>ASAKLPGDFGPPRGEPIHAVLTSPPLVPPPVNRTYPAKVIVELEVVEKEMQISEGVSYTFWTFGGTVPGSFIRVRQGDTVEFHLKNHPSSKMPHNIDLHGVTGPGGGAASSFTAPGHESQFTFKALNEGIYVYHC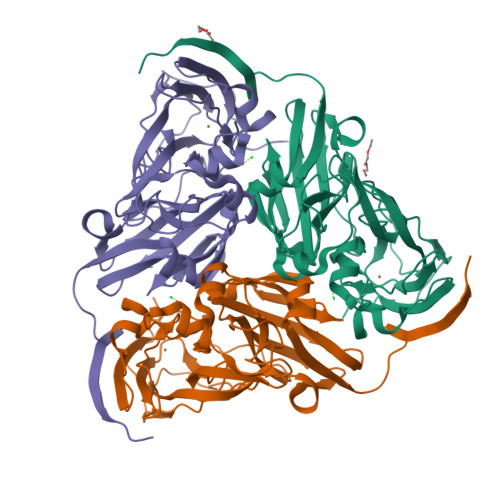ATAPVGMHIANGMYGLILVEPPEGLPKVDHEYYVMQGDFYTAGKYREKGLQPFDMEKAIDERPSYVLFNGAEGALTGDKALHAKVGETVRIFVGNGGPNLVSSFHVIGAIFDQVRYEGGTNVQKNVQTTLIPAGGAAVVKFTARVPGSYVLVDHSIFRAFNKGAMAILKIDGAENKLVYSGKELDSVYLGDRAAPN[6x]> MGSSHHHHHHMTYEYILVRYGEMTTKGKNRSKFVSTLKDNVKFKLKKFPNIKIDATHDRMYIQLNGEDHEAVSERLKDVFGIHKFNLAMKVPSELEDIKKGALAAFLQVKGDVKTFKITVHRSYKHFPMRTMELLPEIGGHILENTEDITVDVHNPDVNVRVEIRSGYSYIMCDERMGAGGLPVGVGGKVMVLLSGGIDSPVAAYLTMKRGVSVEAVHFHSPPFTSERAKQK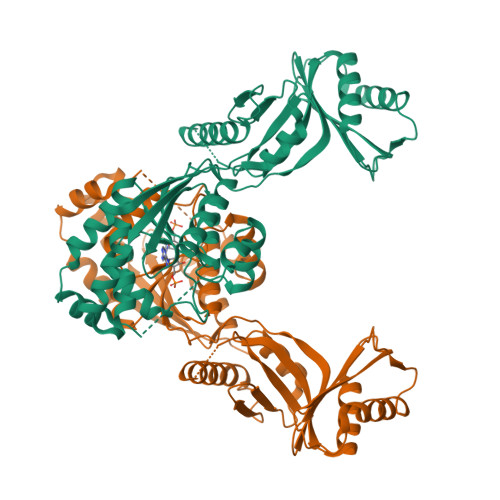VIDLAQELTKYCKRVTLHLVPFTEVQKTINKEIPSSYSMTVMRRMMMRITERIAEERNALAITTGESLGQVASQTLDSMHTINEVTNYPVIRPLITMDKLEIIKIAEEIGTYDISIRPYEDCCTVFTPASPATKPKREKANRFEAKYDFTPLIDEAVANKETMVLQTVEVVAEEEKFEELF Chromatin remodeling complex NoRC (nucleolar remodeling complex) interacts with the rDNA promoter regions of silent genes repressing rDNA transcription. It consists of TIP5 (TTF-I interacting protein 5), also known as BAZ2A (bromodomain [BRD] adjacent to zinc finger domain protein 2A), which is the largest subunit, and the adenosine triphosphatase (ATPase) SNF2h (sucrose nonfermenting protein 2 homologue). BAZ2B shares 29% sequence identity with TIP5 at the full-length level and harbors similar domain organization. Both proteins contain a MBD (methyl-CpG-binding domain), also known as TAM (TTF-IIP5, ARBP, MeCP1) domain, AT-hook DNA-binding domains, DDT (DNA binding homeobox and different transcription factors), and a PHD (plant homeodomain) zinc finger adjacent to a BRD at their C terminus. Our crystal structures combined with biophysical and mutagenesis data demonstrate that PHD zinc fingers recognize N-terminal unmodified H3K4 tail, whereas the TIP5 and BAZ2B BRDs recognize H4K16ac and H3K14ac, respectively, with specificity pattern KacXXR.

In order to compare the molecular mechanism of the recognition of these sites, we solved high-resolution crystal structures of TIP5 and BAZ2B BRDs with histone H4 peptides bearing acetylation marks at K8, K12, and K16. In contrast to H3K14ac and H4K16ac, the diacetylated peptide H4(6–13)K8acK12ac simultaneously bound two BAZ2B BRD molecules in the complex crystal structure that was solved at 1.6 Å resolution. Interestingly, in this dual-recognition binding mode, the segment H4(6–10) containing the K8ac mark targets one BRD molecule, whereas the H4(10–13) is recognized by a second BRD module. The linking residue L10 may favor the crystallographic packing in its well-accommodated hydrophobic cage formed by F2139 by each BRD. ITC measurements also confirmed a 2:1 stoichiometry of protein to peptide, hence two N-acetyl lysine binding sites for a single histone tail with two acetylation marks. Although this complex is unlikely to be physiological, structural data suggest that BAZ2B BRD recognize only single lysine acetylation marks per binding site.

>[2x]SMDSKDLALCSMILTEMETHEDAWPFLLPVNLKLVPGYKKVIKKPMDFSTIREKLSSGQYPNLETFALDVRLVFDNCETFNEDDSDIGRAGHNMRKYFEKKWTDTFK;> GKGLGKG> GVLRSLYSRVSQRVWSTLHFRVGSRGQVRTNKGFKPTAFPHLG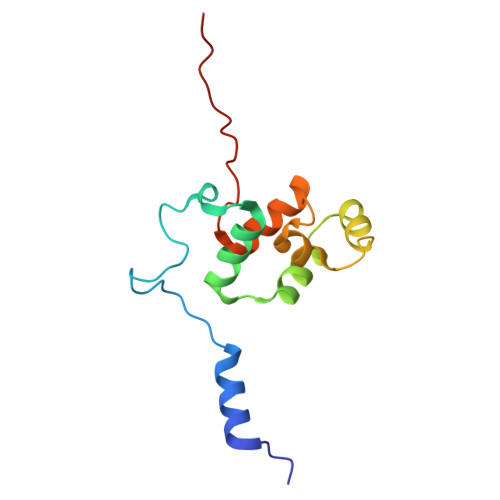AALFFARMSKGLTRDSVEKFVRLNVSEAQRQEIKNWPGSVVRCIENGACIPSRELQSRLEQVVGVPLTRRKKRAGNRRL> GPLGSMQRINNAIDSLIGHLVPAAAGDDDDARTRRQAVFDLVRALLEQPGSNIPSDVNHASDLIKRRLISTNPSQALRFSNLYTRLLALPVLNQKWAILYLLHQLAD;> GPHMPPSERAEKQAAAQQAVDILHEIATILNCHLDRRTLSICISMIENGVNPEALANVIKELRVL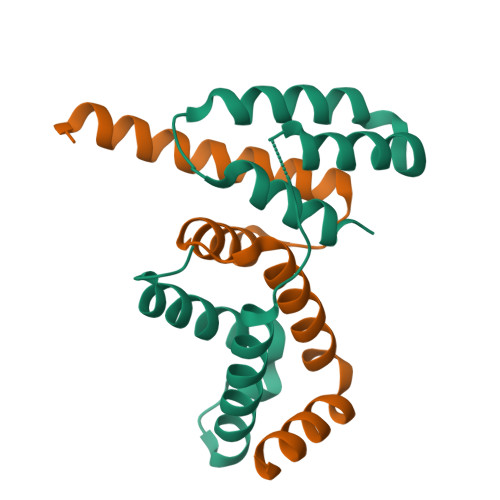GQDPQQLDALVANYLASSRRR> FANFF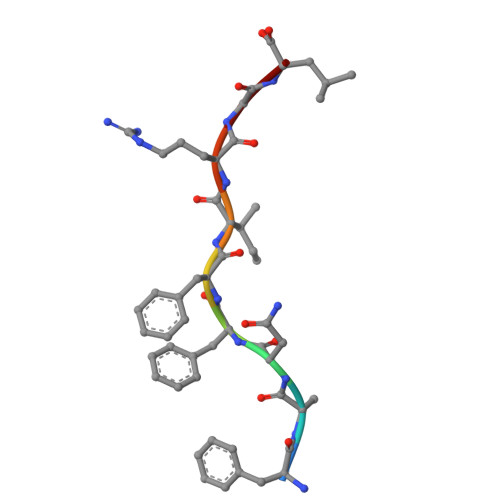IRGL>MGRDPNSSSVDKLAAALEHHHHHHMSAVASHVVPPRSKLDSILSSGLEHNIDHDPLEVWDKGVFLNELLKQGIALSTNENGTLDGELVADEGLKKGSYKGTRLALTEIYSILEDAAVSHFDKRGYEPIFPVKRELDLKKRIYQWSDGTDGYPPHLKVDGNDEANLPADERQSKPGSARSEGVGQIFDMQETAFVSKIAQAVSFIIPKDIDHENTPYKGPTLADVEKFNKAQFPKTDGDASNQDNLNKAADIMKGRNIGEYDDWYSDARFAQQHFSGVNPSTIETASQDKIKEYISEAQKQGLDKVKAILEDGKDILIQDYSYFREATGATNEQIFQNTVYELKGTTPTGKTTSRYAAASVVIFQLHEDGRLHPLAITLDYKGSLDNSITIFNRRLSPDDTCDIAEKEDWPWRYAKTVAQTADWARHEVATHLVDTHMIEEAIIVATNRIIPEGELLYEILSPHWFRTLSLNAAARKLLVPGVIARIAGFGPTSPSLDFKGNNAFKLIDWSYKNFNFQDKYIPNDLKKRGFDIKGDKSGKYKNYPYANDMYLLWGIIRNFVKTVIESQYTSDHVVQKDPYIGGWCKEIQTNGQIPTFPTITTVEQLIDAVTMCIHTASPQHTAVNYLQDYYYSFVPAKPPALCTPLPQDLSALQGYTEKDLTAA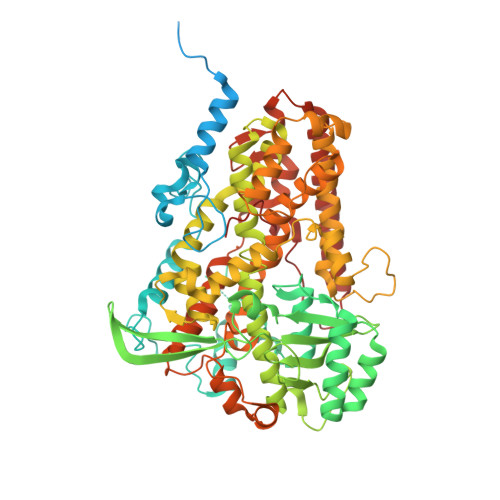LPIGTEDMKWKDWLLAAQLPELLSYKVQQDYNLITYAKSLYNVNKNRTITENTKFNCKTIKKAAADFYSHLKSAGVEFENYSKGQTAGTVEYPVLQPETTAISILI[2x]> GSNFCDSKCKLRCSKAGLADRCLKYCGICCEECKCVPSGTYGNKHECPC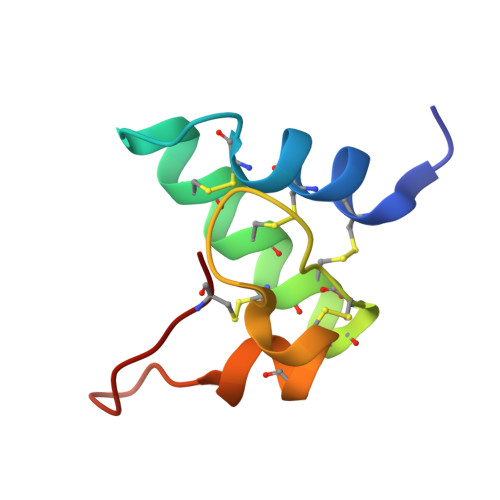YRDKKNSKGKSKCP>HPIEVVLRDMNNKDARQKIKDEVNTQKEGKFRLTIKRDIRNVLSLRVLVNGTFLKHPNGDKSLSTLHRLNAYDQNGGLVAKLVATDDLTVEDEKDGHRILNSLFERFDEGHSKPIRAAET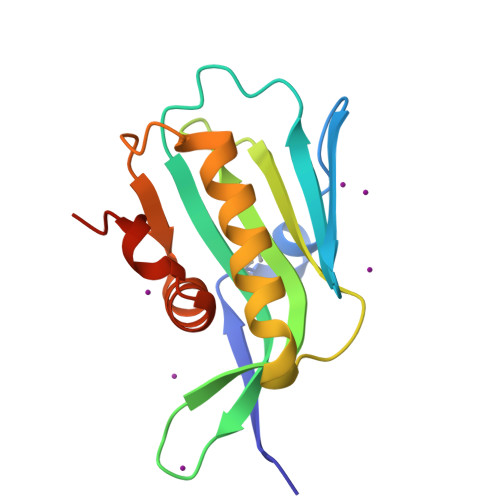AVGVLSQFGQEHRLSPEEGDN[2x]> SRERIVPVVYYLSRNGRLDHPHFIEVPLSSHNGLYLKDVINRLNDLRGNGMACLYSWSSKRTYKNGFVWYALSDEDFIFPVHGQEYVLKGSQILD

We recently discovered Arabidopsis SOSEKI proteins, which exhibit polar localization throughout development. Polar localization of SOSEKI proteins involves two conserved domains: a central domain required for membrane association that dictates localization to polar edges, and an N-terminal domain required for focused localization at these edges (Yoshida et al., 2019). Furthermore, we use structural and biochemical analysis to establish that this ancient protein family contains a bona fide DIX domain—constituting the closest structural relatives of the Dishevelled DIX domain—and that these domains, like Dishevelled DIX, undergo concentration-dependent head-to-tail polymerization. Concentration-dependent polymerization via a bona fide DIX domain allows these to recruit ANGUSTIFOLIA to polar sites, similar to the polymerization-dependent recruitment of signaling effectors by Dishevelled.

Note that no structure of a wild-type (WT) Dishevelled DIX has been determined as yet, although multiple structures of domains bearing polymerization-blocking point mutations have been solved (Liu et al., 2011, Madrzak et al., 2015, Yamanishi et al., 2019a, Yamanishi et al., 2019b). We thus used the structure of the human Dishevelled-2 (DVL2) DIX domain (Madrzak et al., 2015), to design a set of point mutations in the AtSOK4 domain that are predicted to attenuate its polymerization (see below). Crystallizing several of these mutations, we succeeded in obtaining diffracting crystals for D85A (equivalent to D78A in AtSOK1), which severely attenuates polymerization. We thus solved the structure of this domain at 1.7 Å resolution, following labeling with selenomethionine to determine phasing. Like DVL2 DIX, the AtSOK4 domain adopts a ubiquitin-like fold, with four β-strands and one α-helix. Strikingly, its α-backbone almost perfectly superimposes on that of DVL2 DIX, with a root-mean-square deviation (RMSD) of 1.74 Å. This was rather unexpected, given the limited primary sequence conservation between the two domains (19/93 residues). Like other DIX domains, AtSOK4 DIX forms a helical filament in the crystal, via head-to-tail interactions of individual monomers. The interface between individual monomers exhibits considerable hydrophobicity, and close hydrophobic interactions (e.g., W83-F81, W83-H34, W83-H36, Y84-F37) are likely to be crucial for the DIX-DIX interaction, although hydrogen bonds (e.g., D85-H36) are also likely to contribute (recall that D85 was mutated for structure determination). Nearly all these residues are fully conserved, or even invariant, among land plant DIX domains, suggesting that they are critical in mediating polymerization. By determining the crystal structure of AtSOK4 DIX, we established that this domain is the closest known relative of the DVL2 DIX domain.>[2x]MMEQVCDVFDIYAICACCKVESKNEGKKNEVFNNYTFRGLGNKGVLPWKCNSLDMKYFRAVTTYVNESKYEKLKYKRCKYLNKE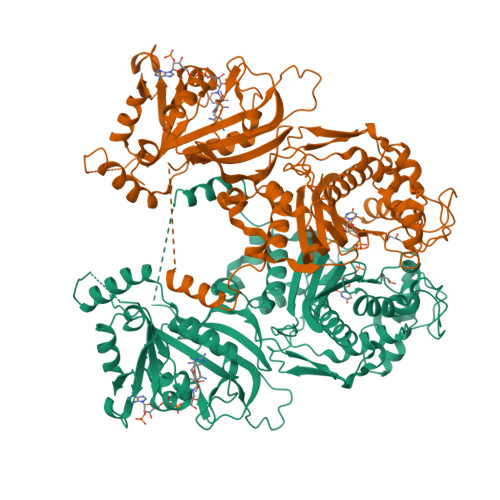TVDNVNDMPNSKKLQNVVVMGRTNWESIPKKFKPLSNRINVILSRTLKKEDFDEDVYIINKVEDLIVLLGKLNYYKCFIIGGSVVYQEFLEKKLIKKIYFTRINSTYECDVFFPEINENEYQIISVSDVYTSNNTTLDFIIYKKTNNKMLNEQNCIKGEEKNNDMPLKNDDKDTCHMKKLTEFYKNVDKYKINYENDDDDEEEDDFVYFNFNKEKEEKNKNSIHPNDFQIYNSLKYKYHPEYQYLNIIYDIMMNGNKQSDRTGVGVLSKFGYIMKFDLSQYFPLLTTKKLFLRGIIEELLWFIRGETNGNTLLNKNVRIWEANGTREFLDNRKLFHREVNDLGPIYGFQWRHFGAEYTNMYDNYENKGVDQLKNIINLIKNDPTSRRILLCAWNVKDLDQMALPPCHILCQFYVFDGKLSCIMYQRSCDLGLGVPFNIASYSIFTHMIAQVCNLQPAQFIHVLGNAHVYNNHIDSLKIQLNRIPYPFPTLKLNPDIKNIEDFTISDFTIQNYVHHEKISMDMAA> EYDYLFKVVLIGDSGVGKSNLLSRFTRN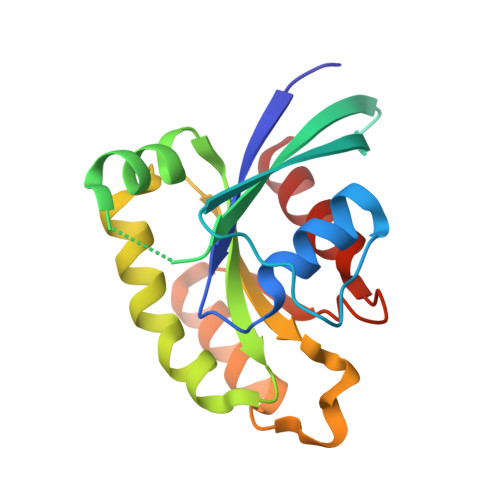EFNLESKSTIGVEFATRSIQVDGKTIKAQIWDTAGQERYRAITSAYYRGAVGALLVYDIAKHLTYENVERWLKELRDHADSNIVIMLVGNKSDLRHLRAVPTDEARAFAEKNGLSFIETSALDSTNVEAAFQTILTEIY Pentameric ligand-gated ion channels (pLGICs) mediate fast chemical signaling between cells. Here, we used the proton-gated ion channel GLIC to identify the conformational changes that occur during gating in the family of pLGIC channels. GLIC has been crystallized in three conformations (called open, closed and locally-closed) and studied by molecular dynamics, normal mode analysis and EPR spectroscopy.

When the bimane is introduced at position 135 (loop B), the pH-fluorescence relationship curve shows an inverted bell-shape, starting after normalization at 0.7, decreasing down to 0.3 at pH 5–4, then increasing up to 0.6 at pH 3. The GLIC structures show a tryptophan (W72 on loop 4) on the same subunit that could play the role of an endogenous quencher. To determine whether W72 has a role in the fluorescence phenotype while avoiding severe mutation-induced structural alteration that would result from the loss of W72, we solved the X-ray structure of Bimane-135 GLIC at pH 4 at 2.6 Å resolution. The structure shows a protein conformation quasi-identical to the wild-type GLIC structure at pH 4 (RMSD = 0.26 Å), with an additional electron density around C135 allowing unambiguous construction of a bimane moiety in two out of the five subunits. The data indeed show that the bimane is at a minimal 3.2 Å distance from the indole ring of W72, which is therefore most likely the major partner in the pH-elicited fluorescence changes of Bimane-135. As the 135 side chain projects at the subunit interface, the quenching of Bimane-135 by W72 seen up to pH 4 suggests a contraction of the domains interfaces, driving the bimane moiety toward W72, although other mechanisms are possible. At very low pH, the bimane appears to move away from the W72. The bimane labeled GLIC V135C was crystallized in the same conditions as WT GLIC. Reflections were integrated using XDS and further processed using programs from the CCP4 suite. As expected, the crystals were isomorphous to the previously described crystal lattice of the open receptor and belonged to space group C121 (unit-cell parameters: a = 182.034 Å, b = 134.075 Å, c = 159.945 Å, α = γ = 90.00°, β = 102.51°) with one pentamer in the asymmetric unit. As the covalent link between the bimane and the cysteine side chain is non-standard, its description was defined in an additional library and incorporated in the pdb file.

>GQDMVSPPPPIADEPLTVNTGIYLIESYSLDDKAETFKVNAFLSLSWKDRRLAFDPVRSGVRVKTYEPEAIWIPEIRFVNVENARDADVVDISVSPDGTVQYLERFSARVLSPLDFRRYPFDSQTLHIYLIVRSCDTRNIVLAVDLEKVGKNDDVFLTGWDIESFTAVVKPANFALEDRLESKLDYQLRISRQYFSYIPNIILPMLFILFISWTAFWSTSYEANVTLVVSTLIAHIAFNILVETNLPKTPYMTYTGAIIFMIYLFYFVAVIEVTVQHYLKVESQPARAASITRASRIAFPVVFLLANIILAFLFFGF[5x]>MGSSHHHHHHSSGLVPRGSHMTDLSDVSRTAAAKPPAVPGRGPANKVRFVTAASLFDGHDASINIMRRILQSQGCEVIHLGHNRSVQEVVTAALQEDVQGIAISSYQGGHVEYFKYMIDLLREHGGEHIQVFGGGGGVIVPDEIRELQAYGVARIYSPEDGQRMGLAGMITDMAQRCDIDLTRYAPTTLDTVVAGDRRALAQLITALENGKADPELVSALHAQAKAAAVPVLGITGTGGAGKSSLTDELIRRFRLDQDDALSIAVISIDPSRRKSGGALLGDRIRMNAINHPNIFMRSLATREAGSEISQALPDVIAACKAARFDLVIVETSGIGQGDAAIVPHVDLSLYVMTPEFGAASALEKIDMLDFADFVAINKFDRKGAQDAWRDVAKQVQRNREQWHSRAEDMPVYGTQASRFNDDGVTMLYQGLVGALGARGMSLKPGTLPNLEGRISTGQNVIVPPARSRYLAELADTVRAYHRRVVAQSKLARERQQLRAAHDMLQGAGHESAALETLASERDVSLGAVERKLLAMWPQMQQAYSGDEYVVKIRDKEIRTGLISTTLSGTKIRKVVLPRFEDEGEILKWLMRENVPGSFPYTAGVFAFKREGEDPTRMFAGEGDAFRTNRRFKLVSEGMEAKRLSTAFDSVTLYGEDPHERPDIYGKVGNSGVSIATLEDMKVLYDGFDLTNPSTSVSMTINGPAPTILAMFMNTAIDQQIDRFRADNGRDPTADEEAKIRAWVLQNVRGTVQADILKEDQGQNTCIFSTEFSLKVMGDIQEYFVHHQVRNFYSVSISGYHIAEAGANPISQLAFTLANGFTYVEAYLARGMHIDDFAPNLSFFFSNGMDPEYSVLGRVARRIWAVTMRDKYGANDRSQKLKYHIQTSGRSLHAQEIDFNDIRTTLQALIAIYDNCNSLHTNAYDEAITTPTAESVRRALAIQLIINREWGVAKCENPNQGSFLIEELTDLVEEAVLQEFERIAERGGVLGAMETGYQRGKIQEESLYYEQLKHDGTLPIIGVNTFRNPNGDPTPQTLELARSSEDEKQSQLHRLTEFHGAHQADAEAMLARLRQAVIDNRNVFAVLMDAVRVCSLGQITHALFEVGGQYRRNM[3x]

Although most chaperones are standalone proteins, isobutyryl-CoA mutase fused (IcmF) has a G-protein domain covalently attached to its target mutase. IcmF catalyzes the 1,2-rearrangement of isobutyryl-CoA to n-butyryl-CoA, as well as pivalyl-CoA and isovaleryl-CoA, using AdoCbl. Here, we show that the G-protein domain in a fused system forms a similar active conformation, requiring IcmF oligomerization. Cryo-EM structural analysis reveals that the second protomer of the G-protein intermolecular dimer props open the mutase active site using residues of switch III as a wedge, allowing for AdoCbl insertion or damaged Cbl removal.

Substituting the switch III residue Q341 with alanine lowers the catalytic efficiency 2.6-fold mainly through a decrease in kcat. To further investigate the structures of IcmF’s supramolecular complexes, we prepared cryogenic EM grids and collected datasets of C. metallidurans wt IcmF with GMPPCP and butyryl-CoA (wt IcmF + GMPPCP) and Q341A IcmF with GTP (Q341A IcmF + GTP). For the Q341A IcmF + GTP dataset, we performed 3D single particle reconstructions, using repeated classifications for both 2D and 3D steps to separate out heterogeneity. Local B factor postprocessing was also performed to yield a 4.6-Å resolution reconstruction. For the Q341A IcmF + GTP reconstruction, there is clear density for the guanosine and at least two phosphates of GTP in all the nucleotide-binding sites. Although the resolution of the cryo-EM IcmF structures is too low for a detailed analysis of protein:G-nucleotide interactions, we do find that the switch III residues including K344 (K188 in MeaB) and Q341 (Q185 in MeaB) of one IcmF protomer are in direct contact with the G-nucleotide bound to another IcmF protomer. Overlaying previously determined closed and open conformations of IcmF onto the structure of Q341A IcmF + GTP reveals that the G-protein interdimer interface clashes with the closed conformation. Specifically, the switch III region (residues 333–344) and a helix (purple in Fig. 7B, residues 363–380) of one protomer clash with two helices of the substrate-binding domain of the other protomer (helix 1, residues 942–965, and helix 2, residues 974–995 in Fig. 7B); these clashes are not observed when the mutase is in an open conformation. Thus, in addition to switch III residues residing at the interface created by the G-protein domains, they also participate in propping open the mutase.3,5-di~{tert}-butylbenzenesulfonamide | C14 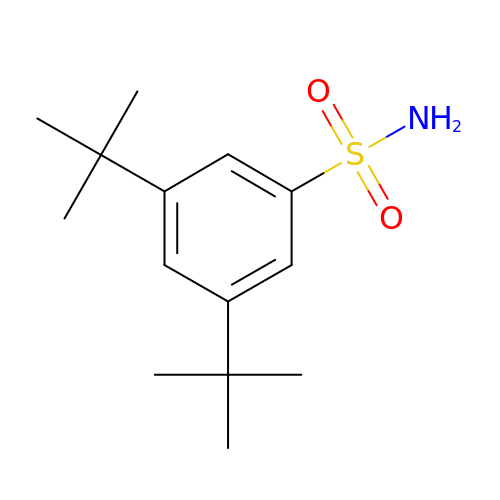H23 N O2 S | JHNRXWPREULLAE-UHFFFAOYSA-N> ARGRRYIGYDALKKNNVPCSRRGRSYYDCKKRRRN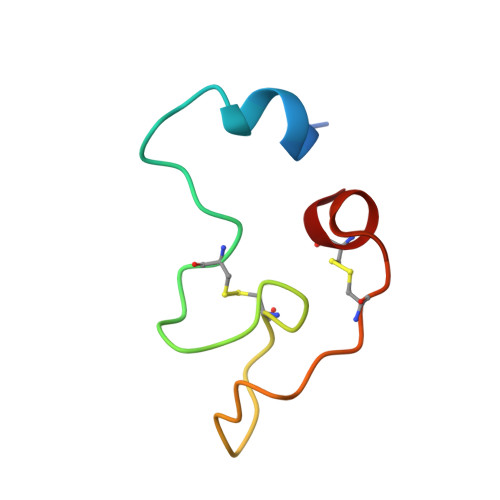NPYRRGCSAITHCYR N-[2-(5-chloro-2-fluorophenyl)pyridin-4-yl]-2-[(piperidin-4-yl)methyl]-2H-pyrazolo[4,3-b]pyridin-7-amine | C23 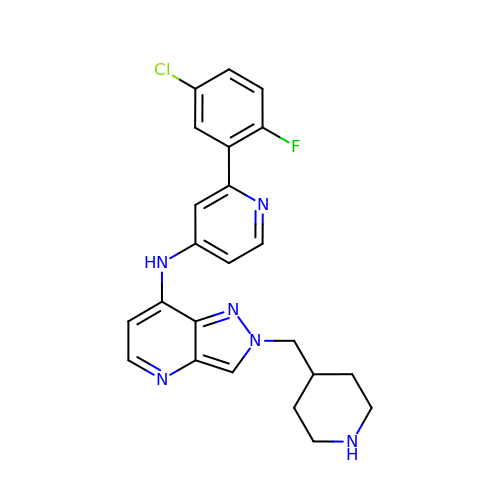H22 Cl F N6 | QZJHLQYMHQMSIQ-UHFFFAOYSA-N>MMELIRIAMKKDLENDNSLMNKWATVAGLKNPNPLYDFLNHDGKTFNEFSSIVNIVKSQYPDREYELMKDYCLNLDVKTKAARSALEYADANMFFEIEDVLIDSMISCSNMKSKEYGKVYKIHRELSNSVITEFEAVKRLGKLNIKTPEMNSFSRLLLLYHYLSTGNFSPMAQLIKQIDLSEISENMYIRNTYQTRVHVLMSNIKLNENSLEECREYSKKALESTNILRFQVFSYLTIGNSL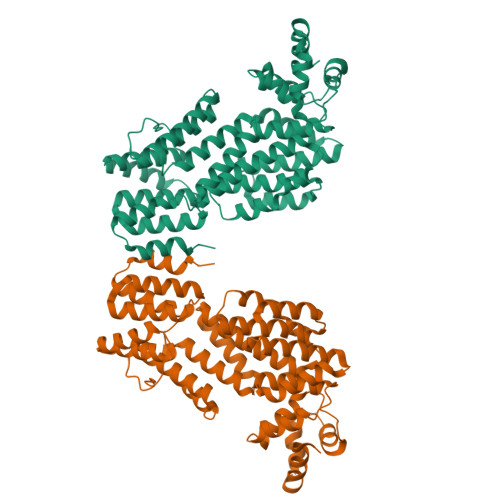LFSNYELAQENFLKGLSISVQNENYNMIFQQALCFLNNVWRKENKWINFESDSIMDLQEQAHCFINFNENSKAKEVLDKLDLLVHNDNELAMHYYLKGRLEQNKACFYSSIEYFKKSNDKFLIRLPLLELQKMGENQKLLELLLLLEHHHHHH[2x]CLC-7 is a member of the CLC family of chloride (Cl-) channels and chloride (Cl-)/proton (H+) transporters and is expressed in the lysosome and the resorption lacuna of osteoclasts. In the membranes of these acidic compartments, CLC-7 uses the large pH gradient to catalyze the uptake of two Cl- ions for each H+ released. Unique among mammalian CLC transporters, CLC-7 requires a β-subunit, osteopetrosis-associated transmembrane protein 1 (OSTM1), for transport activity. In this study, we present structures of the lysosomal Cl-/H+ exchanger CLC-7 alone and in complex with its obligatory β-subunit OSTM1.

Reconstruction of these particle images with twofold symmetry imposed yielded a structure of dimeric ggCLC-7 at a resolution of 2.9 Å that enabled model building. Each protomer of dimeric ggCLC-7 contains a transmembrane domain composed of 18-transmembrane helices and a cytoplasmic domain composed of an N-terminal domain and two C-terminal cystathionine β-synthase (CBS) domains. The second constriction (1.1 Å minimum radius) is at the luminal entrance and is formed by the side chains of Lys242, Glu467 and the backbone of Gly241. Together the three constrictions yield an occluded state for the transporter, sealing off the external and central Cl--binding sites from the cytosol and the lysosomal lumen. In ggCLC-7, the Glugate (Glu243) adopts the ‘up’ conformation, where it participates in establishing one of the luminal constrictions. Within the Cl--conduction pathway, non-protein densities that we attributed to Cl- ions were resolved at the external, central and internal Cl--binding sites. In the ggCLC-7 structure, Gluin (Glu310) on helix αG is located more than 15 Å away from Glugate, where it extends into a solvent filled cavity between the transmembrane and cytosolic domains that is continuous with the cytosol. We modeled this non-protein density as a Mg2+-bound ATP based on its shape and a comparison with the ATP-bound structure of the isolated CBS domains of CLC-5 (Meyer et al., 2007). In particular, both ATP and Mg2+ directly interact with the N-terminal domain of CLC-7. The well-resolved head group allowed us to model the density as a phosphoinositol-3-phosphate (PI3P), which is a low-abundance constituent of lysosomal membranes. In contrast, the alternative conformation adopted by Phe510 in the ggCLC-7 structure widens the pathway sufficiently to allow water molecules to cross (1.4 Å minimum radius).

>[2x]MANVAKKVSWSGRDPRDDEDERAGETTPLLNGTGPGSAGGARQFTPSSFLRPGQLSNVDLNEDIRELETELPRPYPNEIPHNEKLLSLKYESLDYDNSENQLFLEEERRINHAAFRTVEIKRWVICAMIGILTGLVACFIDIVVENLAGLKYRVVKDNIDKFTEKGGLSFSLLLWATLNASVVMVGSVIVAFIEPVAAGSGIPQIKCYLNGVKIPHVVRLKTLVIKVCGVILSVVGGLAVGKEGPMIHSGAVIAAGISQGRSTSLKRDFKIFEYFRRDTEKRDFVSAGAAAGVSAAFGAPVGGVLFSLEEGASFWNQFLTWRIFFASMISTFTLNSVLSVYHGNAWDLSSPGLINFGRFDSEKMGYTIQEIPIFIFMGVVGGILGALFNALNYWLTMFRIRYIHRPCLQVIEAMLVAAVTAAVGFVMIYCSRDCQPIQGSSVAYPLQLFCADGEYNSMATAFFNTPEKSVVNLFHDPPGSYNPMTLGMFTLMYFFLACWTYGLTVSAGVFIPSLLIGAAWGRLFGISLSYLSKGSIWADPGKYALMGAAAQLGGIVRMTLSLTVIMMEATGNVTYGFPIMLVLMTAKIVGDYFVEGLYDMHIQLQSVPFLHWEAPVTSHSLTAREVMSTPVTCLRRIERVGTVVDILSDTSSNHNGFPVVESNPNTTQVAGLRGLILRSQLIVLLKHKVFVERANLNLVQRRLKLKDFRDAYPRFPPIQSIHVSQDERECMIDLSEFMNPSPYTVPREASLPRVFKLFRALGLRHLVVVNNHNEVVGMVTRKDLARYRLGKEGLEELSLAQT6-amino-2-(methylamino)-4-phenethyl-1,7-dihydro-8H-imidazo[4,5-g]quinazolin-8-one 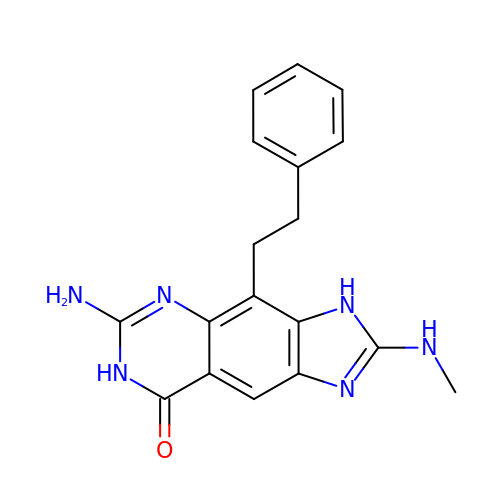| C18 H18 N6 O | WJCDAOMLVZDAIC-UHFFFAOYSA-N> MDPSLVLEQTIQDVSNLPSEFRYLLEEIGSNDLKLIEEKKKYEQKESQIHKFIRQQGSIPKHPQEDGLDKEIKESLLKCQSLQREKCVLANTALFLIARHLNK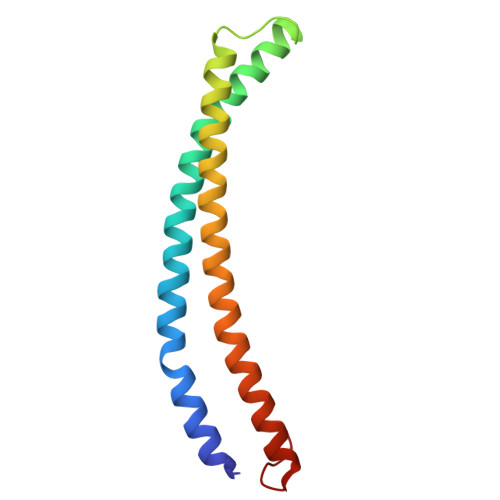LEKNIALLEEDGVLAPV> MVP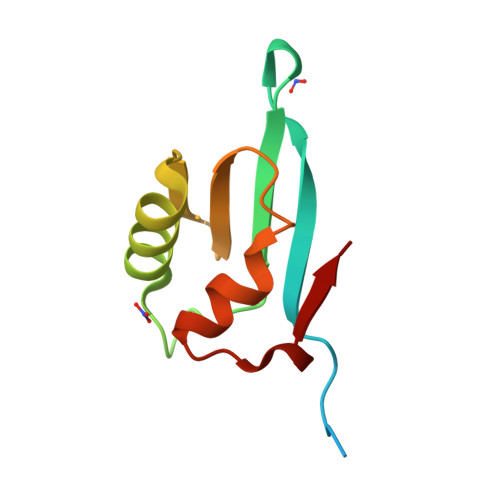RIVNPLDEMLFKEVLKEQQRIKVYIERARYGKVKTIIEGIDEKEFDLEEIAKKLKAKLACGGTAKNGRIELQGDHRDRIKKLLAELGFSEELIEVE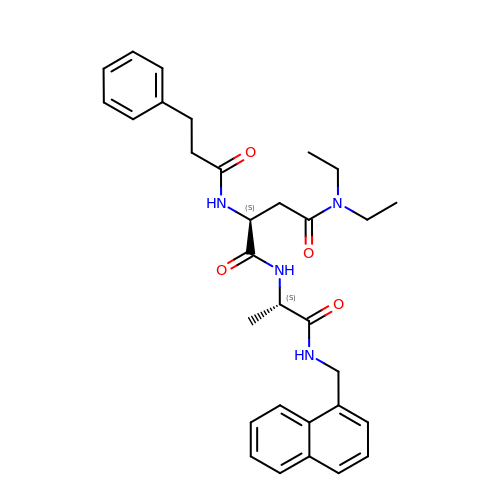N,N-diethyl-N~2~-(3-phenylpropanoyl)-L-asparaginyl-N-[(naphthalen-1-yl)methyl]-L-alaninamide | C31 H38 N4 O4 | PVYXXOWWWHYLGR-CUNXSJBXSA-N> ANPYERGPNPTDALLEASSGPFSVSEENVSRLSASGFGGGTIYYPRENNTYGAVAISPGYTGTEASIAWLGERIASHGFVVITIDTITTLDQPDSRAEQLNAALNHMINRASSTVRSRIDSSRLAVMGHSMGGGGTLRLASQRPDLKAAIPLTPWHLNKNWSSVTVPTLIIGADLDTIAPVATHAKPFYNSLPSSISKAYLELDGATHFAPNIPNKIIGKYSVAWLKRFVDNDTRYTQFLCPGPRDGLFG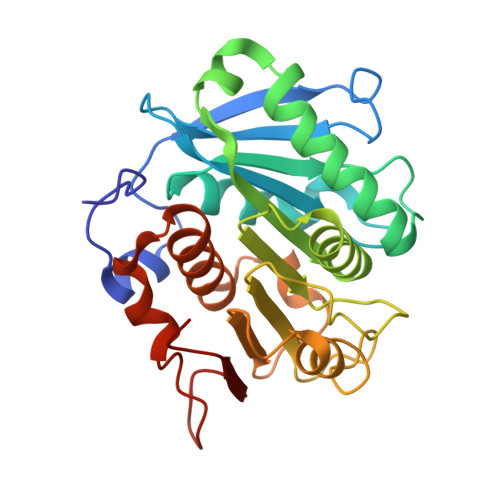EVEEYRSTCPF> PISPIETVPVKLKPGMDGPKVKQWPLTEEKIKALVEICTEMEKEGKISKIGPENPYNTPVFAIKKKDSTKWRKLVDFRELNKRTQDFWEVQLGIPHPAGLKKKKSVTVLDVGDAYFSVPLDEDFRKYTAFTIPSINNETPGIRYQYNVLPQGWKGSPAIFQSSMTKILEPFKKQNPDIVIYQYMDDLYVGSDLEIGQHRTKIEELRQHLLRWGLTTPDKKHQKEPPFLWMGYELHPDKWTVQPIVLPEKDSWTVNDIQKLVGKLNWASQIYPGIKVRQLCKLLRGTKALTEVIPLTEEAELELAENREILKEPVHGVYYDPSKDLIAEIQKQGQGQWTYQIYQEPFKNLKTGKYARMRGAHTNDVKQLTEAVQKITTESIVIWGKTPKFKLPIQKETWETWWTEYWQATWIPEWEFVNTPPLVKLWYQLEKEPIVG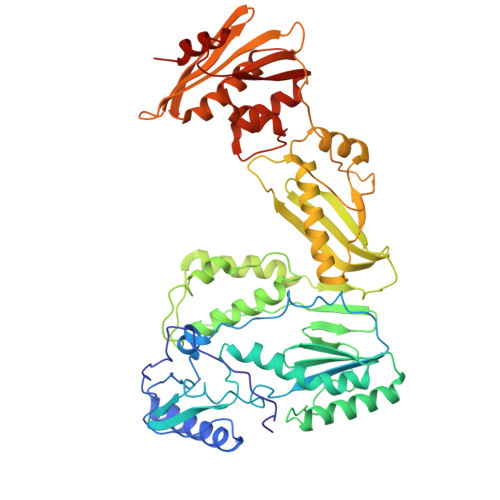AETFYVDGAANRETKLGKAGYVTNKGRQKVVPLTNTTNQKTELQAIYLALQDSGLEVNIVTDSQYALGIIQAQPDKSESELVNQIIEQLIKKEKVYLAWVPAHKGIGGNEQVDKLVSAGIRKIL PTPN21 belongs to the four-point-one, ezrin, radixin, moesin (FERM) domain–containing protein tyrosine phosphatases (PTP) and plays important roles in cytoskeleton-associated cellular processes like cell adhesion, motility, and cargo transport. Because of the presence of a WPE loop instead of a WPD loop in the phosphatase domain, it is often considered to lack phosphatase activity. However, many of PTPN21’s biological functions require its catalytic activity. Combined with biochemical analysis, we have found that PTPN21 PTP is weakly active and is autoinhibited by association with its FERM domain.

To further investigate the working mechanism of the phosphatase domain of PTPN21, we determined structures of PTPPTPN21 C1108S in complex with a phosphate ion as well as PTPPTPN21 C1108S in complex with a Src pY530 peptide. In the 2.0-Å PTPPTPN21 C1108S-Src pY530 peptide complex structure, the electron density of the phosphotyrosine residue and the catalytic water is clearly resolved. The tyrosine moiety is mainly stabilized by hydrophobic packing with F927, A1110, and V1112, and the phosphate group is coordinated by the P loop and R1114. The catalytic water forms hydrogen bonds with the phenolic oxygen as well as Q1152 and Q1156. The WPE loop is in an open conformation despite the bound peptide. Alignment of the peptide-bound open PTPPTPN21 C1108S structure with phosphate-bound closed PTPPTPN21 structure showed that the phosphate ion and the phosphate group of the phosphotyrosine are in a nearly identical position, so is R1114, despite around 10-Å shift of the WPE loop. Furthermore, E1067 in the closed structure is within steric clash distance (1.9 Å) with the tyrosine moiety in the open structure, further indicating that the closed structure might represent a conformation after P─O bond cleavage. When a phosphotyrosine substrate is present, for catalysis to happen, E1067 would have to move to a certain position between the open and closed conformations currently observed. Close examination of the electron density revealed that C1155-C1070 in the open structure formed a disulfide bond, while C1155 and C1070 in the WPE closed structure are free with a distance around 3.9 Å. It is possible that the open conformation promoted C1155-C1070 disulfide bond formation which prevented the WPE loop from clamping down.

> TRATNDERCKILEQRLEQGMVFTEYERILKKRLVDGECSTARLPENAERNRFQDVLPYDDVRVELVPTKENNTGYINASHIKVSVSGIEWDYIATQGPLQNTCQDFWQMVWEQGIAIIAMVTAEEEGGREKSFRYWPRLGSRHNTVTYGRFKITTRFRTDSGCYATTGLKMKHLLTGQERTVWHLQYTDWPEHGCPEDLKGFLSYLEEIQSVRRHTNSTSDPQSPNPPLLVHSSAGVGRTGVVILSEIMIACLEHNEVLDIPRVLDMLRQQRMMLVQTLCQYTFVYRVLIQFLKSSRLI;> EPQYQ CYTIDINE-5'-TRIPHOSPHATE | C9 H16 N3 O14 P3 | 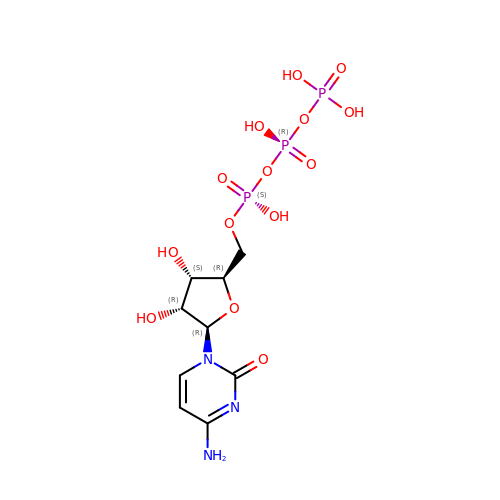PCDQPRRSZKQHHS-XVFCMESISA-N> MSEDKAKLGTTRSATEYRLSIGSAPTSRRSSMGESSSLMKFADQEGLTSSVGEYNENTIQQLLLPKIRELSDSIITLDSNFTRLNFIHESLADLNESLGSLLYGIMSNSWCVEFSQAPHDIQDDLIAIKQLKSLEDEKNNLVMELSNMERGIKRKKDEQGENDLAKASQNKQFNQPLFPSSQVRKYRSYDNRDKRKPSKIGNNLQVENEEDYEDDTSSEASFVLNPTNIGMSKSSQGHVTKTTRLNNNTNSKLRRKSILHTIRNSIASGADL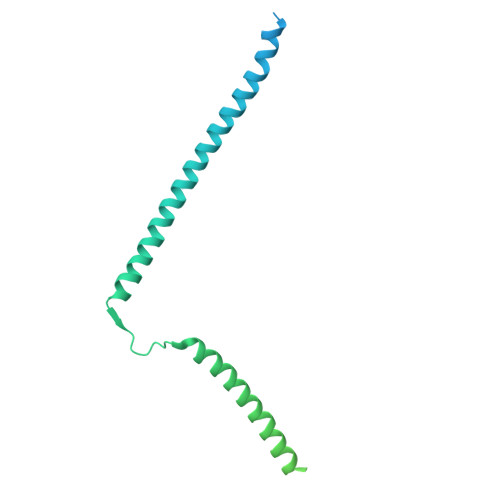PIENDNVVNLGDLHPNNRISLGSGAARVVNGPVTKNRNSMFSGRAERKPTESRHSVAKKTEKKINTRPPFR> CTCSPSHPQDAFCNSDIVIRAKVVGKKLVKEGPFGTLVYTIKQMKMYRGFTKMPHVQYIHTEASESLCGLKLEVNKY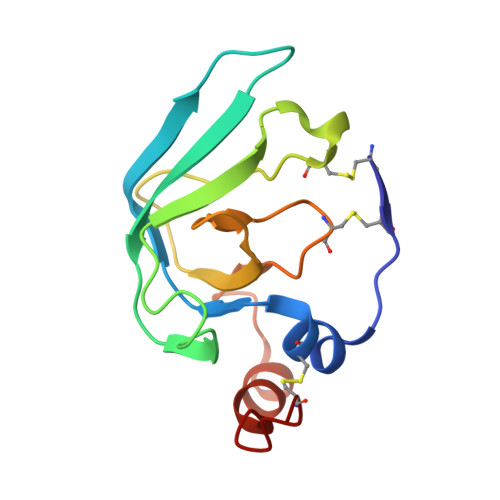QYLLTGRVYDGKMYTGLCNFVERWDQLTLSQRKGLNYRYHLGCN> DVSGTVCLSALPPEATDTLNLIASD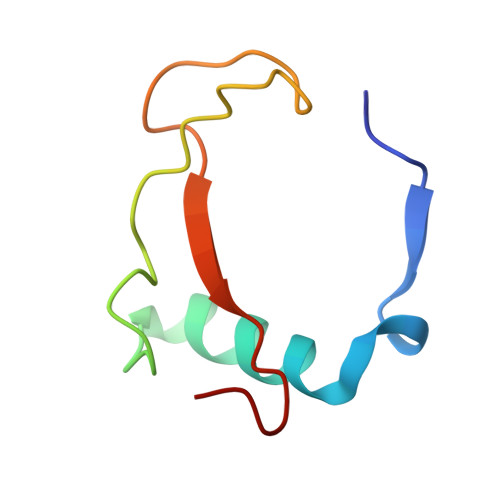GPFPYSQDGVVFQNRESVLPTQSYGYYHEYTVITPGAR> MAAGSRFPFCTAARLSSRGTLPRLGEATFFAGAESQRSAGAFAKTLQRPFLRAPSTQLFPVGNRLGVSSARALVANAMEPRRFFAAAASAKATHALQPTGTGSVAFTRPGQGSNAQFQT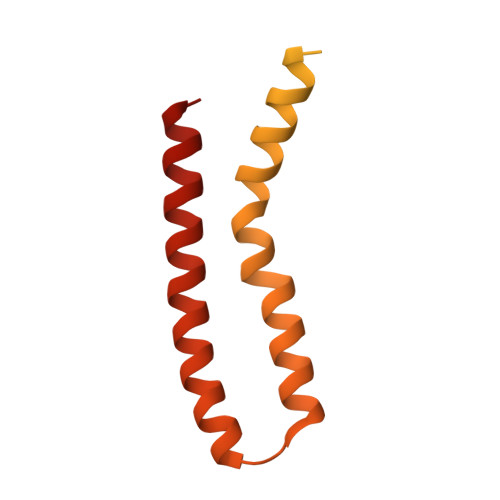SLADKTRGLLGVGFLRPTKMASFAATFLLNFRFYFMYMARTTFQAVRPLLAFSVFGEVMKLVLATMSSGLFSFLFSFVLAFEVFYFFLQCYISYTFLTMFFTVLF> GRCT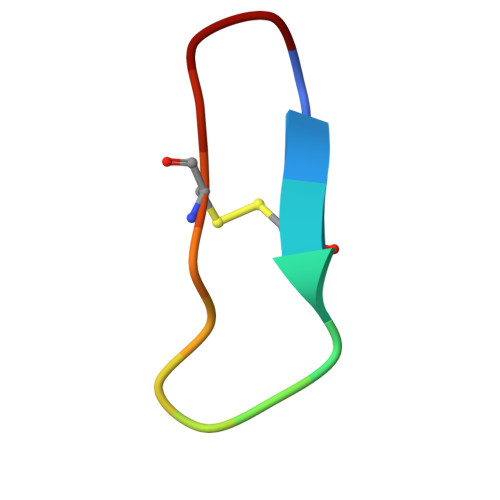KSIPPICFPD>SASAVEDIRKVLSDSSSPVAGQKYDYILVGGGTAACVLANRLSADGSKRVLVLEAGPDNTSRDVKIPAAITRLFRSPLDWNLFSELQEQLAERQIYMARGRLLGGSSATNATLYHRGAAGDYDAWGVEGWSSEDVLSWFVQAETNADFGPGAYHGSGGPMRVENPRYTNKQLHTAFFKAAEEVGLTPNSDFNDWSHDHAGYGTFQVMQDKGTRADMYRQYLKPVLGRRNLQVLTGAAVTKVNIDQAAGKAQALGVEFSTDGPTGERLSAELAPGGEVIMCAGAVHTPFLLKHSGVGPSAELKEFGIPVVSNLAGVGQNLQDQPACLTAAPVKEKYDGIAISDHIYNEKGQIRKRAIASYLLGGRGGLTSTGCDRGAFVRTAGQALPDLQVRFVPGMALDPDGVSTYVRFAKFQSQGLKWPSGITMQLIACRPQSTGSVGLKSADPFAPPKLSPGYLTDKDGADLATLRKGIHWARDVARSSALSEYLDGELFPGSGVVSDDQIDEYIRRSIHSSNAITGTCKMGNAGD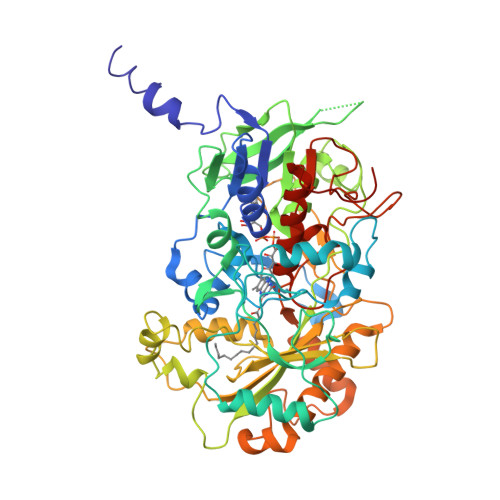SSSVVDNQLRVHGVEGLRVVDASVVPKIPGGQTGAPVVMIAERAAALLTGKATIGASAAAPATVAA[6x]> DPISNAIENAVSTLADTTISRVTAANTAASSHSLGTGRVPALQAAETGASSNASDENLIETRCVMNRNGVNEASVEHFYSRAGLVGVVEVKDSGTSQDGYTVWPIDVMGFVQQRRKLELSTYMRFDAEFTFVSNLNDSTTPGMLLQYMYVPPGAPKPDGRKSYQWQTATNPSIFAKLSDPPPQVSVPFMSPASAYQWFYDGYPTFGEHKQATNLQYGQCPNNMMGHFAIRTVSESTTGKNVHVRVYMRIKHVRAWVPRPFRSQAYMVKNYPTYSQTISNTAADRASITTTDYEGGVPANPQRTF;> SPSVEACGYSDRVAQLTVGNSTITTQEAANIVLSYGEWPGYCPSTDATAVDKPTRPDVSVNRFYTLSTKSWKTESTGWYWKFPDVLNDTGVFGQNAQFHYLYRSGFCMHVQCNASKFHQGALLVVVIPEFVVAASSPATKPNGQGLYPDFAHTNPGKEGQVFRDPYVLDAGIPLSQALVFPHQWINLRTNNCATIIMPYVNALPFDSALNHSNFGLAVIPISPLKYCNGATTEVPITLTIAPLNSEFSGLRQAIKQ;> GLPTELKPGTNQFLTTDDGTSPPILPGFEPTPLIHIPGEFTSLLDLCRIETILEVNNTTGTTGVNRLLIPVRAQNNVDQLCASFQVDPGRNGPWQSTMVGQICRYYTQWSGSLKVTFMFTGSFMATGKMLIAYTPPGSAQPTTREAAMLGTHIVWDFGLQSSVTLVIPWISNTHFRAVKTGGVYDYYATGIVTIWYQTNFVVPPDTPSEANIIALGAAQENFTLKLCKDTDEIRQTAEYQN

Coxsackievirus A6 (CV-A6) has recently overtaken enterovirus A71 and CV-A16 as the primary causative agent of hand, foot, and mouth disease worldwide. To initiate infection, enterovirus particles progress through a set of distinct functional intermediates: the infectious native virion expands into a destabilised altered or A-particle, in which the internal capsid protein VP4 has been displaced. The genome is released through a capsid opening, leaving the empty capsid as the non-infectious end product. The major capsid proteins VP1, VP2, and VP3 are arranged with pseudo-T = 3 icosahedral symmetry with VP1 subunits forming pentamers around the fivefold axes and VP2 and VP3 forming heterohexamers around the threefold symmetry axes of the capsid.

The structure of the CV-A6 virion was determined to a resolution of 2.68 Å, whereas those of the altered and empty particles reached resolutions of 2.50 and 2.82 Å, respectively. The structures of the altered and empty particles of CV-A6 are similar, and the capsid proteins forming their icosahedral asymmetric units can be superimposed with an r.m.s.d. of 0.31 Å for 633 of 638 Cα atoms available for the comparison. The buried surface area of 4400 Å2 per protomer within the altered capsid is less than half than that of the virion. Like the previously studied enteroviruses, the conversion of CV-A6 virions to the altered particles is connected to the loss of ordered structures of VP4 subunits and the N- and C-termini of the major capsid proteins, but also of surface loops of VP1, VP2, and VP3. The structures of the altered particle and the virion of CV-A6 can be superimposed with an r.m.s.d. of 0.82 Å for 548 Cα atoms of 659 available for the comparison. The centre of mass of the protomer in the expanded altered particle is 135 Å from the particle centre, whereas it is 130 Å in the virion. Moreover, the core of VP1 in the altered particle is positioned closer to VP2 and VP3 than in the virion. The GH loop of VP1 (residues 205–214), the EF loop of VP2 (139–143), and the GH loop of VP3 (175–186) are structured in the virion but not in the altered particle. Residues 45–47 from the N-terminal AB loop of VP2 form a short α-helix located near the twofold symmetry axis of the altered particle, whereas in the empty particle these residues are disordered. Because of its position, the α-helix may stabilise the altered particle prior to genome release.4-amino-4-deoxy-1-O-[(S)-hydroxy{[(2E,6E,10Z,14Z,18Z,22E,26E,30E)-3,7,11,15,19,23,27,31,35-nonamethylhexatriaconta-2,6,10,14,18,22,26,30,34-nonaen-1-yl]oxy}phosphoryl]-alpha-L-arabinopyranose 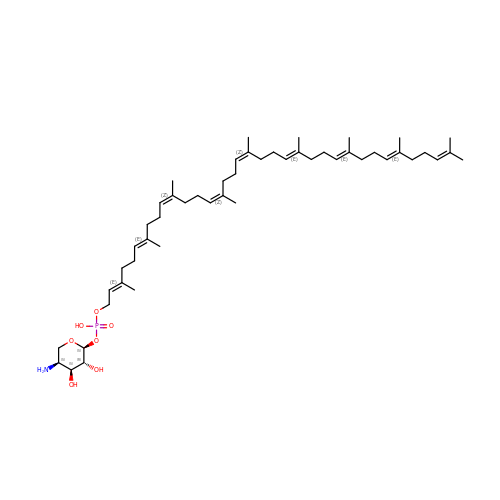| C50 H84 N O7 P | GWCJFQXZVUXOPR-BFSVMLBVSA-N4-CARBOXY-5-(1-PENTYL)HEXYLSULFANYL-1,2,3-TRIAZOLE 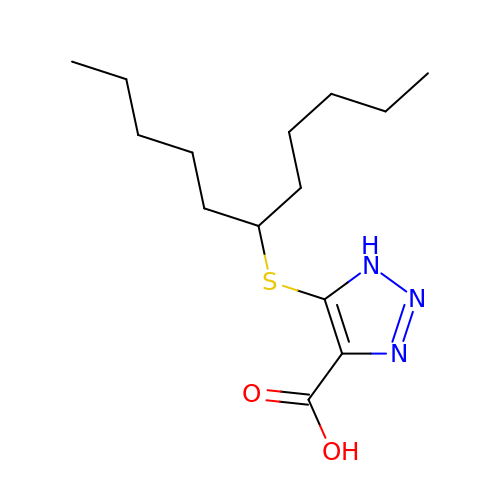| C14 H25 N3 O2 S | GROSWUGUHPUYIU-UHFFFAOYSA-N>IRCFITPDITSKDCPNGHVCYTKTWCDAFCSIRGKRVDLGCAATCPT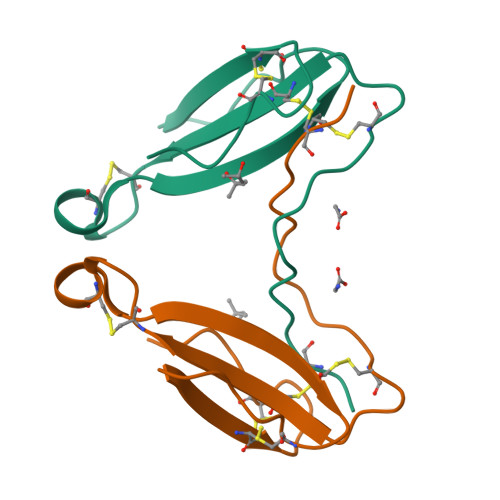VKTGVDIQCCSTDNCNPFPTRKRP[2x]>[2x]MNSVIETILNHRSIRKYEDKPLSEEQIQTIVESAQAASTSSYIQAYSIIGVKDKETKRKLAQLAGNQPYVETNGHFFVFCADFHRHDVIAEMEKKDLSTALESTEQFMVAIIDVALAAQNATLAAESMGLGACYIGGLRNELEEVSKLLKLPHHVIPLFGLTVGHPAGIT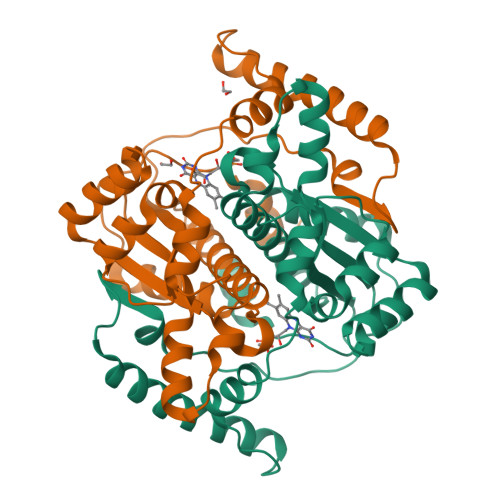DKKPRLPFKHVYHEETYEPNDEQTKKELTAYNEEISAYYNERTNGKRQDTWTGQMAEMLSNPKRMYMKEFVEKQGFNKKKGHHHHHH> EVDKRREINNEHPLLMMPLYANGEEFNQGKYTFWGGDTLTGKWENIPDDLKPYTVIQLHPDDLPKRDGAARDFYEHMLEEAAKYVNPKTGKNEPIPVILTVYTAGNMPYHTSAHWLSTSWIDKMYQKYPNLHGIFSTASYWIWANDIENKAADYLKVSAKNGGYFIWAEQNSGSAIEKAFGKNGKIAFQKSVDKYWKNLIFMFKNTPAAEGNDST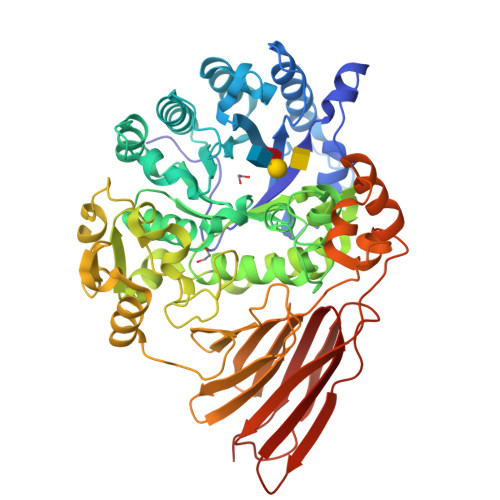TESYMKGLWLSNHTYQWGGLMDTWKWYETGKWKLFASGNIGKSQGDRQWLTEPESMLGEEALGVYLNGGVVYNFEHPAYTYGVNNKESLLFSEVIKEFFRYVIAHPAPSKEKVLEDTKVFIHGDYSNKGNGKFFVNVNTDREQTPLYMTGRYNVIPAIPGVLKTDKLKESVSSSRIQIKEITSPEFSSTQARKEYLNKLYPMNYEGDIFAQKLDNRWFVYNYKVNENVKQTGKLKFNSLEMNVEFEPHTYGIFERISNGLKVNLNNFRTNKDSLWSNAQDANQAKKLPQLTKKGAIKWIEEHYIKDTQFGEKRVTKIVLRGIDKLPTIHSLSGTNNSYDQPSLNFDQKNHMVTITINSNGNLEFELHFLEHPPPPPLRSGC>MALADISGYLDVLDSVRGFSYLENAREVLRSGEARCLGNPRSEPEYVKALYVIGASRIPVGDGCSHTLEELGVFDISVPGEMVFPSPLDFFERGKPTPLVRSRLQLPNGVRVWLKLEWYNPFSLSVADRPAVEIISRLSRRVEKGSLVADATSSNFGVALSAVARLYGYRARVYLPGAAEEFGKLLPRLLGAQVIVDPEAPSTVHLLPRVMKDSKNEGFVHVNQYYNDANFEAHMRGTAREIFVQSRRGGLALRGVAGSLG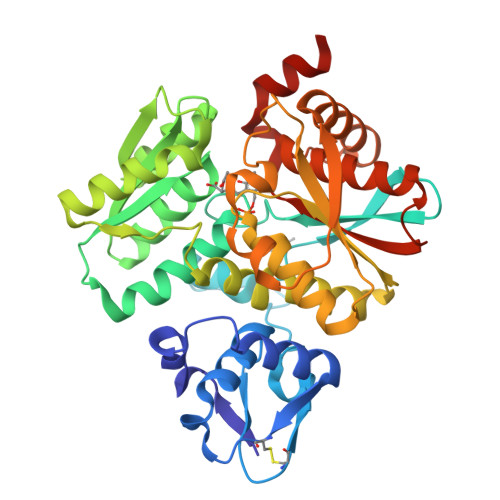TSGHMSAAAFYLQSVDPSIRAVLVQPAQGDSIPGIARVETGMLWINMLDISYTLAEVTLEEAMEAVVEVARSDGLVIGPSGGAAVKALAKKAAEGDLEPGDYVVVVPDTGFKYLSLVQNALEGAGDSV[4x]> MKNTTTYDYIVVGGGTSGLVVANRLSENP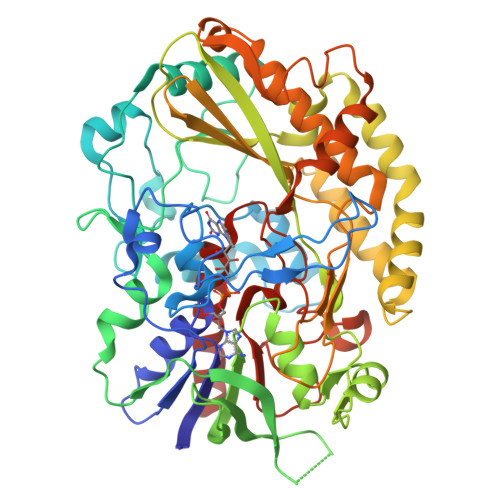DVSVLLLEAGASVFNNPDVTNANGYGLAFGSAIDWQYQSINQSYAGGKQQVLRAGKALGGTSTINGMAYTRAEDVQIDVWQKLGNEGWTWKDLLPYYLKSENLTAPTSSQVAAGAAYNPAVNGKEGPLKVGWSGSLASGNLSVALNRTFQAAGVPWVEDVNGGKMRGFNIYPSTLDVDLNVREDAARAYYFPYDDRKNLHLLENTTANRLFWKNGSAEEAIADGVEITSADGKVTRVHAKKEVIISAGALRSPLILELSGVGNPTILKKNNITPRVDLPTVGENLQDQFNNGMAGEGYGVLAGASTVTYPSISDVFGNETDSIVASLRSQLSDYAAATVKVSNGHMKQEDLERLYQLQFDLIVKDKVPIAEILFHPGGGNAVSSEFWGLLPFARGNIHISSNDPTAPAAINPNYFMFEWDGKSQAGIAKYIRKILRSAPLNKLIAKETKPGLSEIPATAADEKWVEWLKANYRSNFHPVGTAAMMPRSIGGVVDNRLRVYGTSNVRVVDASVLPFQVCGHLVSTLYAVAERASDLIKEDAKSA> AQSVPYGVSQIKAPALHSQGYTGSNVKVAVIDSGIDSSHPDLKVAGGASFVPSETNPFQDNNSHGTHVAGTVAALDNSIGVLGVAPSASLYAVKVLGADGSG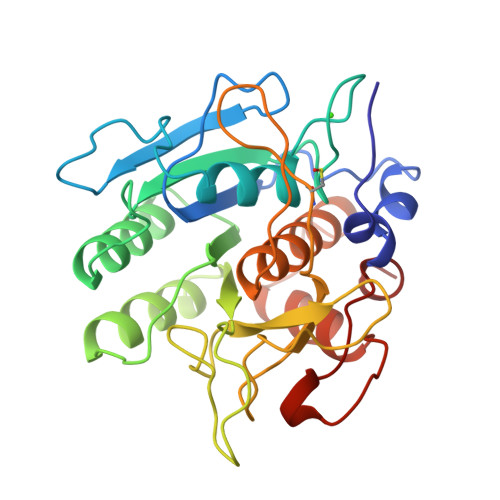QYSWIINGIEWAIANNMDVINMSLGGPSGSAALKAAVDKAVASGVVVVAAAGNEGTSGSSSTVGYPAKYPSVIAVGAVDSSNQRASFSSVGPELDVMAPGVSICSTLPGNKYGAYSGTSMASPHVAGAAALILSKHPNWTNTQVRSSLENTTTKLGDSFYYGKGLINVQAAAQ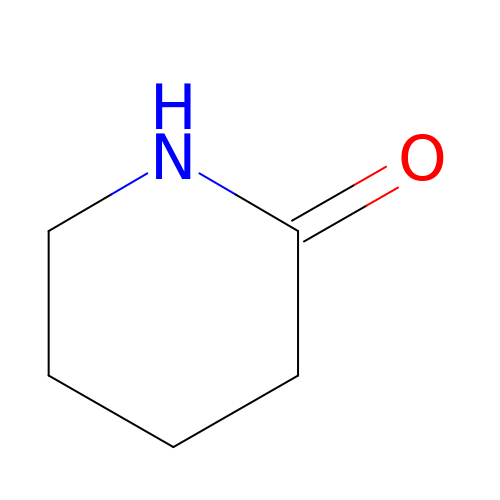piperidin-2-one | C5 H9 N O | XUWHAWMETYGRKB-UHFFFAOYSA-N>[2x]MPRKKDQVTKNDDGNQTSDVQTQDFKTAVQPDTNTAQLIKTYSNPKQRGDKGEIIYDGGLSSKLADVVDKTTEPHNADGAVKDGRIAPVKLDLEKQKLDKLKLFETSPFDPLTIKNNQDVVDKLYATQSSSIQEVVPTKTFATELQFGVTSEDMAKIYGAVAAVSKNVNSSVTYEVKRGTHELIKVPTIPHNLVLIQSDNGKHALIKEDLGQWPVETGISLVNQAGVFAVQLANKLGIDKPFVLDAGSNYFTDTSFIDTRKYCTDGLSPREIQKALNRQRAYYDRPELTISENKTLLSQSIIYPDADGNDVSIIFSGAMSHAIFTYAQSQWNKNIIKLDDYIREITLTVPKQYRPRRFKEIEHTHGYVYRELNQGSLLPLVDANLKESSSYYFKKLMSSISNVPVDARTLQSATAALAADTGQAVNRAQHVSMLTNRLTTANAPTVRAITVLTCMFKQFRIGMTYALDPNIMDVAAATCMLLFRPAQSISDEQYRYCLQTMAVFLTNTTYDIVNNDTIDVLKMKLRNQGWPFVERYNAVEIDMSVEPLRSPGQVGRYYNPFNIDPLTKKHVEDRLEEFINQVQVGRFRNASGNAVGTTLAAFLRACRDKTSANWRGYSVLVSRYRSLIPNELFESLRNISGEYNINPQDEHSFFFALAQINADDEFIGAIDKESAEYLDEYATLARDISNSLTLVKAAFGPLERTSGSIINHANNLNKVINHVFADKPLISETMLKILTIDGTTGKDGYRNWLDKLVGHNYPVYVEPVVNIMNFISARFVADSSYFGYTNEIMIMPNHINVPVDDRFGFRDSPFCTSLPRTIMGNDVRRISYNVFSMMEDIDDVISEGFILYDAYFNFSYDIMTTDGVTRLKEDILIVTDTGNDIKPIHFYIYFENRNDKKLRYESKMNVSYRLYIKTPACLLPLSDYMRAQHDYVSPSSSRVYIKDPAVVYTRS;>[13x]MANRATSAFLDNPHPVGVNYVDEGSRQFVAVAELLASKLIDSSRESDESNSDVPFVQAYSKFADDNPRHLRVKTGGKMANALTNVIRSYYSINAPAIVPQVEIDRLASKATVSGDMYNSYAIFNSVPIVEVLSPARTTVSIVGSDRADVTMLNTGAGAANITFNFGQIAETVILKGSVPFQLARLNQPMPAARFTYKLRPLDGPFIVVLPVGNPLVISATAATRIQVPLAFNKALVESGFQTAMNDGLFDIQNVNYYSSFDEFIISQYHAQDGINRVSTCVILGLALQAYDQMRRALPVRRV;>MDVLSKGSLKELLAHLEKTPLEEAISYRIGTVPYQNVLISRNEYYNQLYPDTTSLIDGVSREGQRNVNGLIMSIISYVVSGSGHYIPNIGFMLLRRSILDILTKHDTGLVTNNLNYGIIARNLTVSKMNCEQRKRMLICFKLLAYKDGNQNDYEIYLNQNIPLKQIAPNFIPGDMRTVIHNQDQLAIVGIPAYRLTQSTELSIRDDNAKSYKLGYVDWYNSNSFLRERSEFNLIRLKDRDTKYGKLNGW[2x];>[3x]MAWVTQAYSSGLSQNSIISLTGNDRTVADGTFNSMIMPRAVIANEREHFMKTRIDKIEHDLNRSAKQEMMDRQSLAEDYNALNLAVGQEIKLDIATQHQLNRLGSAMYKADHERETELTDLINRIRENEVTVNGILENQKAITAAERADLLLEVVASTAKSVSAAGRAAADGSGVVPVFGPSVANGIKVGIDIADSVAEAAIAVKESGIITQLNDVYHAFQSV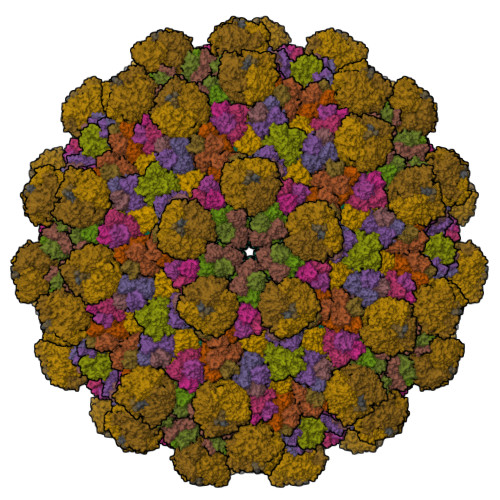HVAPNDVIKPAAVVAGTSTELIGNLQAIYSRLRSHSDIGFKKATVGDVIPNSYMIKPVNSTEYASWQLYVIHPVQGSLGLVVQLMGDALTYNVFAQYGNTSASEFGKTVLTGGATNTALEGTKVKFQTKVTAQQALALTMALKDAASMLSQGELIGYFEQYINLALEPDNLSLQDNMHKYHHLLTSQNSPIDWNYHDEEMHKWLDSRKTTNYDAMQKKDGTVIADIHIPKVFNDLRNTTLHCKLEGKQTIAGYTVYEYLIGPWAHYGDIDYSVVVDTLNEETKWYCEVIGIDGHLLIEKSVQHKPEKILELTVNDSGVTSFNGRNHDRLKLKVYVKDSLSVKVFRNWIGINAPRVKTKMFNDHIGVKYDYSHFDKNISPAHLTLTDLGWHTWDQYNAGNWTNIKP;>MLSETELRALKKLSTTTSRVVGDSTLALPSNVKLSKGEVEKIAVTKKEMFDELAQCNLPTIELITREHTFNGDVIRFAAWLFLMNGQKLMIANNVAVRMGMQYATNLAGNNVKITYVTSNNVVKLGHIAAGVLANPYSNKGSGLFITYEYNLISNLIETGKVCVLFITSLSTTASSTNSFAYSTCSVPIENWDFNMIKLTAETSCASLTAMTNLVNSLVPGERTRPVGLYVDIPGVTVTTSASSGSLPLTTIPAVTPLIFSAYTKQVEEVGVINTLYALSYLP[3x]>NLIKQLQERGLVAQVTDEEALAERLAQGPIALVCGFDPTADSLHLGHLVPLLCLKRFQQAGHKPVALVGGATGLIGDPSFKAAERKLNTEETVQEWVDKIRKQVAPFLDFDCGENSAIAANNYDWFGNMNVLTFLRDIGKHFSVNQMINKEAVKQRL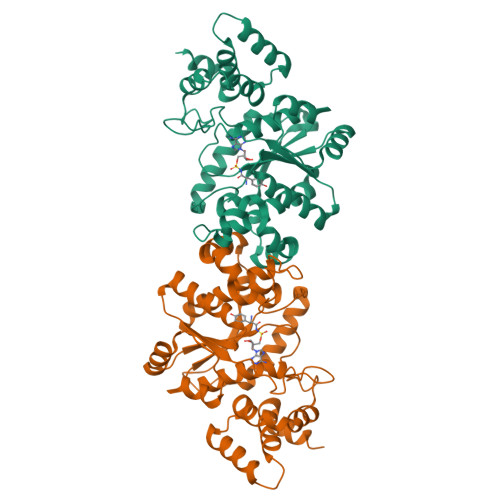NREDQGISFTEFSYNLLQGYDFACLNKQYGVVLCIGGSDQWGNITSGIDLTRRLHQNQVFGLTVPLITKADGTKFGKTEGGAVWLDPKKTSPYKFYQFWINTADADVYRFLKFFTFMSIEEINALEEEDKNSGKAPRAQYVLAEQVTRLVHGEEGLQAAKR[2x]>GHMEIDPKDLTFLKELGTGQFGVVKYGKWRGQYDVAIKMIKEGSMSEDEFIEEAKVMMNLSHEKLVQLYGVCTKQRPIFIITEYMANGCLLNYLREMRHR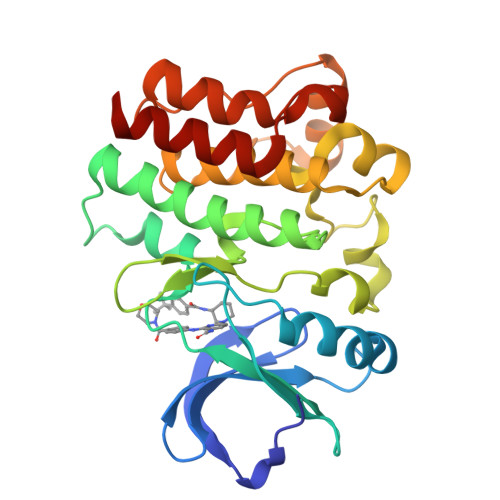FQTQQLLEMCKDVCEAMEYLESKQFLHRDLAARNCLVNDQGVVKVSDFGLSRYVLDDEYTSSVGSKFPVRWSPPEVLMYSKFSSKSDIWAFGVLMWEIYSLGKMPYERFTNSETAEHIAQGLRLYRPHLASEKVYTIMYSCWHEKADERPTFKILLSNILDVMDEES[2x]> MFQQLSARLQEAIGRLRGRGRITEEDLKATLREIRRALMDADVNLEVARDFVERVREEALGKQVLESLTPAEVILATVYEALKEALGGEARLPVLKDRNLWFLVGLQGSGKTTTAAKLALYYKGKGRRPLLVAADTQRPAAREQLRLLGEKVGVPVLEVMDGESPESIRRRVEEKARLEARDLILVDTAGRLQIDEPLMGELARLKEVLGPDEVLLVLDAMTGQEALSVARAFDEKVGVTGLVLTKLDGDARGGAALSARHVTGKPIYFAGVSEKPEGLEPFYPERLAGRILGMGDIESILEKVKGLEEYDKIQKKMEDVMEGKGKLTLRDVYAQIIALRKMGPLSKVLQHIPGLGIMLPTPSEDQLKIGEEKIRRWLAALNSMTYKEL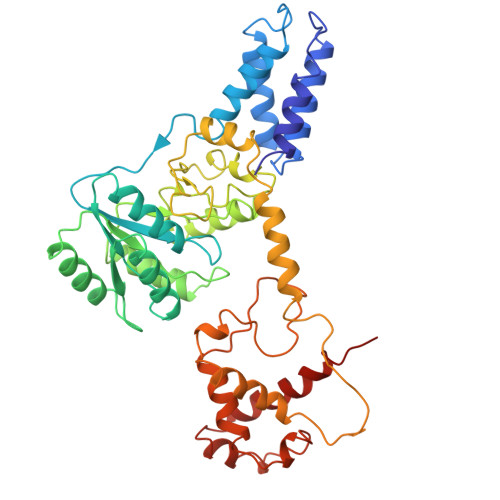ENPNIIDKSRMRRIAEGSGLEVEEVRELLEWYNNMNRLLKMVK> GPHMPGSGQIQLWQFLLELLS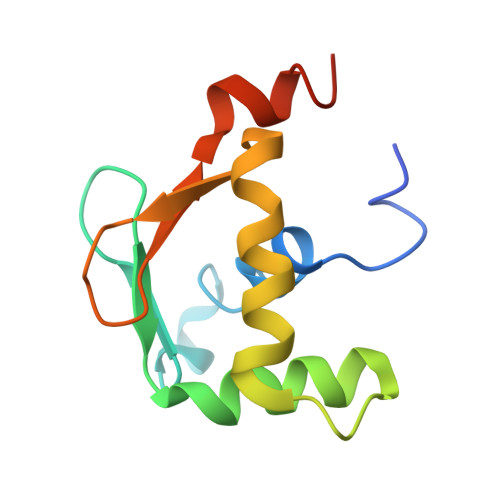DSANASCITWEGTNGEFKMTDPDEVARRWGERKSKPNMNYDKLSRALRYYYDKNIMTKVHGKRYAYKFDFHGIAQALQPHPTE> MFELVDNIAQTAVIKVIGVGGGGGNAVNHMAKNNVEGVEFICANTDAQALKNIAARTVLQLGPGVTKGLGAGANPEVGRQAALEDRERISEVLEGADMVFITTGMGGGTGTGAAPIIAEVAKEMGILTVAVVTRPFPFEGRKRMQIADEGIRALAESVDSLITIPNEKLLTILGKDASLLAAFAKADDVLAGAVRGISDIIKRPGMINVDFADVKTVMSEMGMAMMGTGCASGPNRAREATEAAIRNPLLEDVNLQGARGILVNITAGPDLSLGEYSDVGNIIEQFASEHATVKVGTVIDADMRDELHVTVVATGLGAR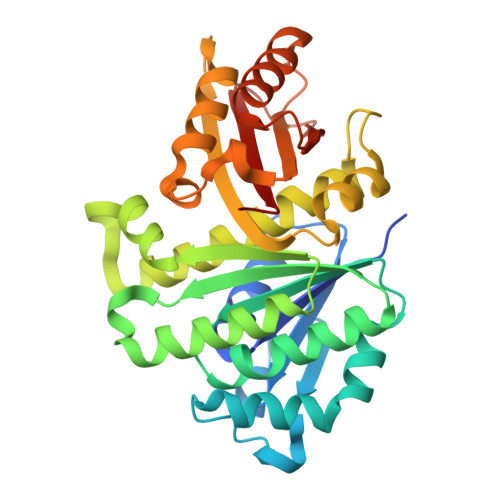L> MADKLFINALKKKFEESPEEKKTTFYTLGGWKQSERKTEFVNAGKEVAEKRGIPQYNPDIGTPLGQRVLMPYQVSTTDTYVEGDDLHFVNNAAMQQLWDDIRRTVIVGLNHAHAVIEKRLGKEVTPETITHYLETVNHAMPGAAVVQEHMVETHPALVADSYVKVFTGNDEIADEIDPAFVIDINKQFPEDQAETLKAEVGDGIWQVVRIPTI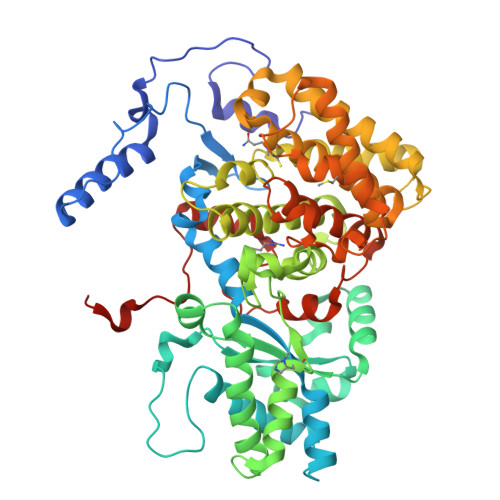VSRTCDGATTSRWSAMQIGMSMISAYKQAAGEAATGDFAYAAKHAEVIHMGTYLPVRRARGENEPGGVPFGYLADICQSSRVNYDDPVRVSLDVVATGAMLYDQIWLGSYMSGGVGFTQYATAAYTDNILDDFTYFGKEYVEDKYGLCEAPNTMDTVLDIATEVTFYGLEQYEEYPALLEDQFGGSQRAAVVAAAAGCSTAFATGNAQTGLSGWYLSMYLHKEQHSRLGFYGYDLQDQCGASNVFSIRGDEGLPLELRGPNYPNYAMNVGHQGEYAGISQAPHAARGDAFVFNPLVKIAFADDNLVFDFTNVRGEFAKGALREFEPAGERALITPAK>MLIAIEGVDGAGKRTLVEKLSGAFRAAGRSVATLAFPRYGQSVAADIAAEALHGEHGDLASSVYAMATLFALDRAGAVHTIQGLCRGYDVVILDRYVASNAAYSAARLHENAAGKAAAWVQRIEFARLGLPKPDWQVLLAVSAELAGERSRGRAQRDPGRARDNYERDAELQQRTGAVYAELAAQGWGGRWLV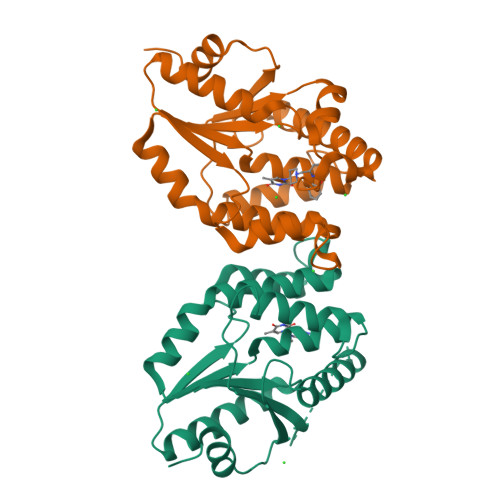VGADVDPGRLAATLAPPDVPS[2x]>[2x]MQMMTRKVLLNMELEEDDDEDGDIVLENFDQTIVCPTFGSLENQQDFRTPEFEEFNGKPDSLFFTDGQRRIDFILVYEDESKKENNKKGTNEKQKRKRQAYESNLICHGLQLEATRSVSDDKLVFVKVHAPWEVLCTYAEIMHIKLPLKPNDLKTRSPFGNLNWFTKVLRVNESVIKPE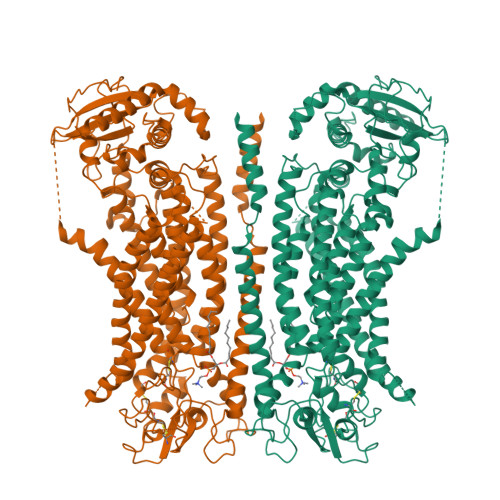QEFFTAPFEKSRMNDFYILDRDSFFNPATRSRIVYFILSRVKYQVMNNVNKFGINRLVSSGIYKAAFPLHDCRFNYESEDISCPSERYLLYREWAHPRSIYKKQPLDLIRKYYGEKIGIYFAWLGYYTQMLLLAAVVGVACFLYGYLDQDNCTWSKEVCDPDIGGQILMCPQCDRLCPFWRLNITCESSKKLCIFDSFGTLIFAVFMGVWVTLFLEFWKRRQAELEYEWDTVELQQEEQARPEYEAQCNHVVINEITQEEERIPFTTCGKCIRVTLCASAVFFWILLIIASVIGIIVYRLSVFIVFSTTLPKNPNGTDPIQKYLTPQMATSITASIISFIIIMILNTIYEKVAIMITNFELPRTQTDYENSLTMKMFLFQFVNYYSSCFYIAFFKGKFVGYPGDPVYLLGKYRSEECDPGGCLLELTTQLTIIMGGKAIWNNIQEVLLPWVMNLIGRYKRVSGSEKITPRWEQDYHLQPMGKLGLFYEYLEMIIQFGFVTLFVASFPLAPLLALVNNILEIRVDAWKLTTQFRRMVPEKAQDIGAWQPIMQGIAILAVVTNAMIIAFTSDMIPRLVYYWSFSIPPYGDHTYYTMDGYINNTLSVFNITDFKNTDKENPYIGLGNYTLCRYRDFRNPPGHPQEYKHNIYYWHVIAAKLAFIIVMEHIIYSVKFFISYAIPDVSKITKSKIKREKYLTQKLLHESHLKDLTKNMGIIAERIGGTVDNSVRPKLE>[2x]RSPWLYCQKGLSMTVEADPANMFNWTTEEVETCDKGALCQETILIIKAGTETAILATKGCIPEGEEAITIVQHSSPPGLIVTSYSNYCEDSFCNDKDSLSQFWEF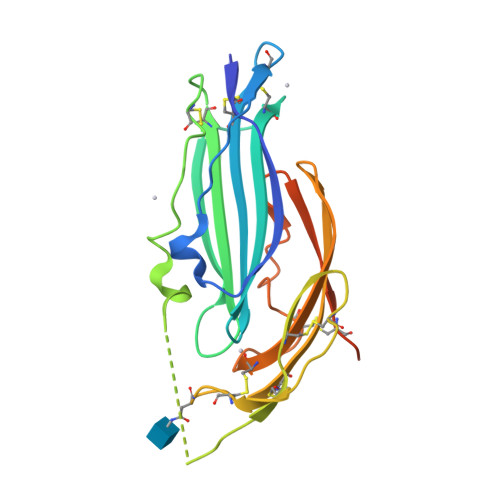SETTASTVSTTLHCPTCVALGTCFSAPSLPCPNGTTRCYQGKLEITGGGIESSVEVKGCTAMIGCRLMSGILAVGPMFVREACPHQLLTQPRKTENEFLEVLFQ PIPERIDIN-2-IMINE | C5 H10 N2 | 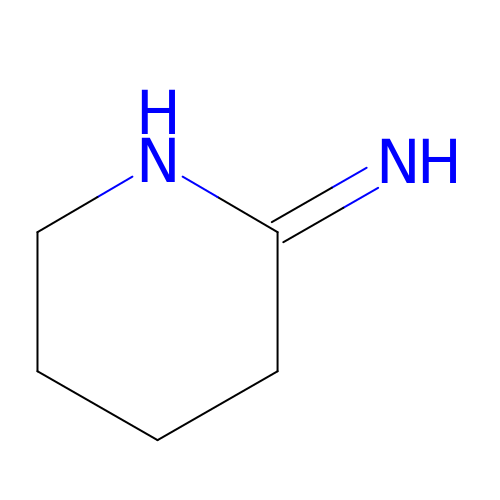DHGUMNJVFYRSIG-UHFFFAOYSA-N>MASMTGGQQMGRDEAGITGTWYNQLGSTFIVTAGADGALTGTYESAAGKAESRYVLTGRYDSAPATDGSGTALGWTVAWKNNYRNAHSATTWSGQYVGGAEARINTQWLLTSGATEANGWASTLVGHDTFTKVKPSAA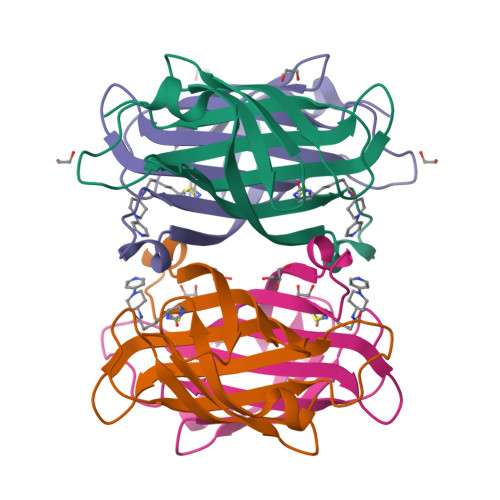SIDAAKKAGVNNGNPLDAVQQ[2x]> GMIKPSNYQPPYTITPAIVNLVAEIGEIIGRYTVLAEQNLTPRLRRENRIRTIQASLAIENNTLTLEQVTAVIDGKRVLGHPREIQEVRNAFATYEAMEDWDASVEGDLLAAHELLMRGLVDETGRYRSGGVGIFRGEQLVHMAPPADRVPKLMADLLDWLENTNEHPLVASCIFHYEFEFIHPFADGNGRMGRLWQTLILRNWKPLLAYLPVETVIRDRQEDYYRVLAVADSQADATPFVEFMLGALRDAVREAVSTDHVGDQVTDQVAALIRAIGGGELSSNDLMQA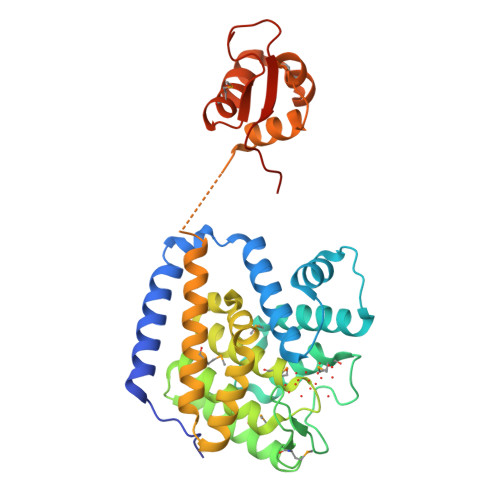LGLSHRPTFRNNYLNPAMEDEWIERTQPDSPRSPTQRYRLTGKGQRWLQHHADE>[2x]IDCGHVDSLVRPCLS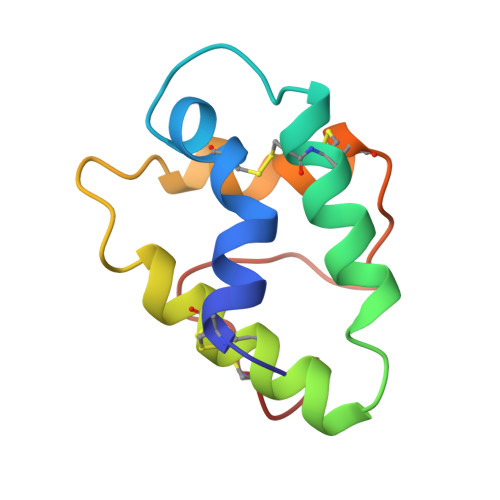YVQGGPGPSGQCCDGVKNLHNQARSQSDRQSACNCLKGIARGIHNLNEDNARSIPPKCGVNLPYTISLNIDCSRV methyl 4-[[4-[[3-[4-(aminomethyl)phenyl]-2-methyl-7-oxidanylidene-pyrazolo[4,3-d]pyrimidin-6-yl]methyl]-4-oxidanyl-piperidin-1-yl]methyl]-3-chloranyl-benzoate 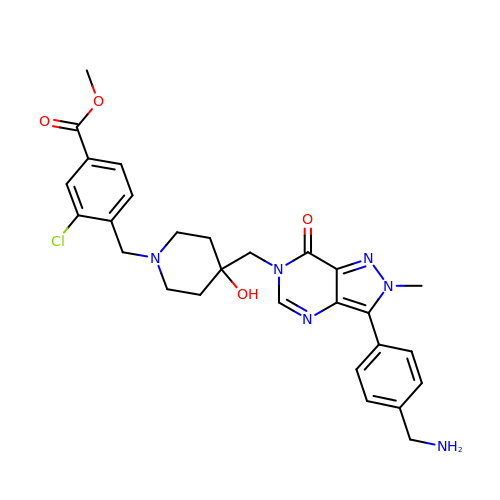| C28 H31 Cl N6 O4 | AQZDRXXVFOYWHG-UHFFFAOYSA-N> KETAAAKFERQHLDS;> NYCNQMMKSRNLTKDRCKPVNTFVHESLADVQAVCSQKNVACKNGQTNCYQSYSTMSITDCRETGSSKYPNCAYKTTQANKHIIVACEGN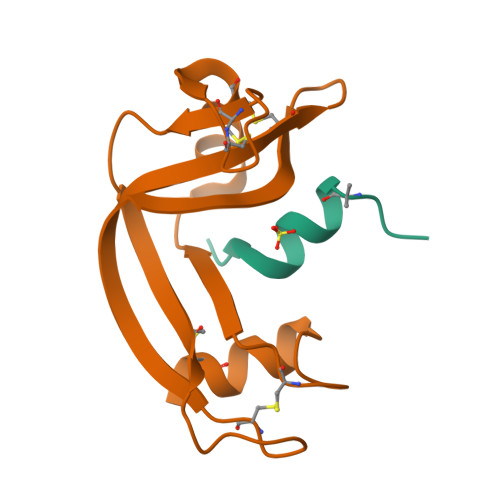PYVPVHFDASV> QN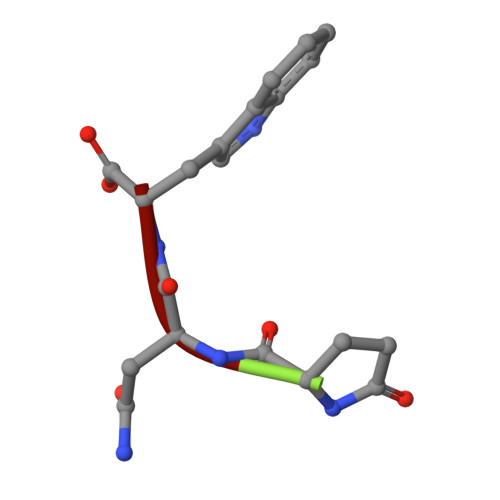W>[2x]MAASMARRLWPLLTRRGFRPRGGCISNDSPRRSFTTEKRNRNLLYEYAREGYSALPQLDIERFCACPEEAAHALELRKGELRSADLPAIISTWQELRQLQEQIRSLEEEKAAVTEAVRALLANQDSGEVQQDPKYQGLRARGREIRKELVHLYPREAQLEEQFYLQALKLPNQTHPDVPVGDESQARVLHMVGDKPVFSFQPRGHLEIGEKLDIIRQKRLSHVSGHRSYYLRGAGALLQHGLVNFTFNKLLRRGFTPMTVPDLLRGAVFEGCGMTPNANPSQIYNIDPARFKDLNLAGTAEVGLAGYFMDHTVAFRDLPVRMVCSSTCYRAETNTGQEPRGLYRVHHFTKVEMFGVTGPGLEQSSQLLEEFLSLQMEILTELGLHFRVLDMPTQELGLPAYRKFDIEAWMPGRGRFGEVTSASNCTDFQSRRLHIMFQTEAGELQFAHTVNATACAVPRLLIALLESNQQKDGSVLVPPALQSYLGTDRI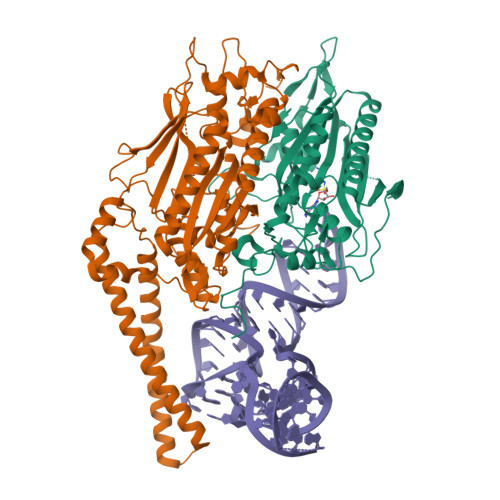TAPTHVPLQYIGPNQPRKPGLPGQPAVS>MVIDSLQLNELLNAGEYKIGELTFQSIRSSQELQKKNTIVNLFGIVKDFTPSRQSLHGTKDWVTTVYLWDPTCDTSSIGLQIHLFSKQGNDLPVIKQVGQPLLLHQITLRSYRDRTQGLSKDQFRYALWPDFSSNSKDTLCPQPMPRLMKTGDKEEQFALLLNKIWDEQTNHSMDPPTFTFNFNNEPWVRGRHETYLCYEVERMHNDTWVKLNQRRGFLANQAPHKHGFLEGRHAELCFLDVIPFWKLDLDQDYRVTCFTSWSPCFSCAQEMAKFISKNKHVSLCIKTARIYDDQGRAQEGLRTLA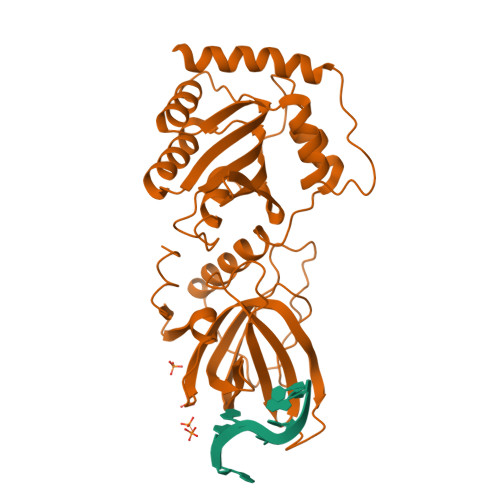EAGAKISIMTYSEFKHCWDTFVDHQGAPFQPWDGLDEHSQDLSGRLRAILQNQEN[4x]Lumacaftor | C24 H18 F2 N2 O5 | 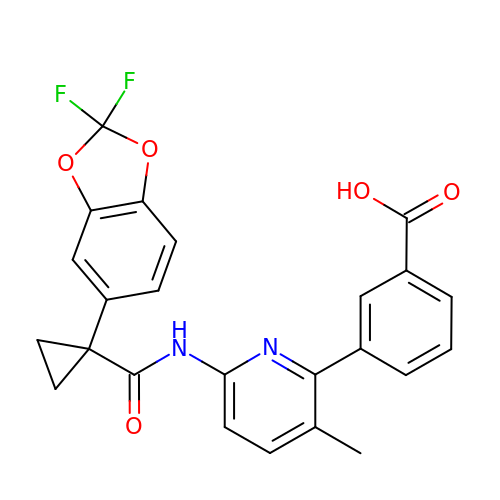UFSKUSARDNFIRC-UHFFFAOYSA-N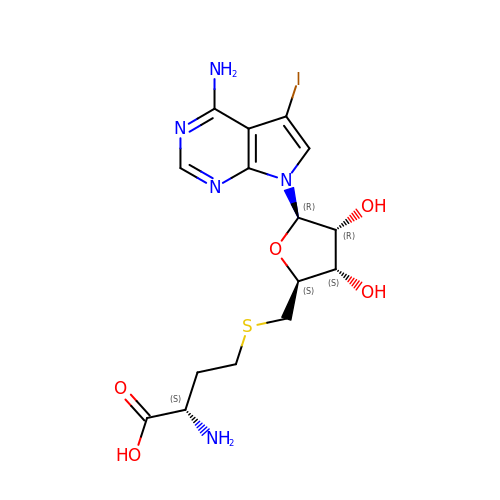(2~{S})-2-azanyl-4-[[(2~{S},3~{S},4~{R},5~{R})-5-(4-azanyl-5-iodanyl-pyrrolo[2,3-d]pyrimidin-7-yl)-3,4-bis(oxidanyl)oxolan-2-yl]methylsulfanyl]butanoic acid | C15 H20 I N5 O5 S | KWPUSSSCXHTEIW-TWBCTODHSA-N>APPSNLMQLPWRQGYSWQPNGAHSNTGSGYPYSSFDASYDWPRWGSATYSVVAAHAGTVRVLSRCQVRVTHPSGWATNYYHMDQIQVSNGQQVSADTKLGVYAGNINTALCEGGSSTGPHLHFSLLYNGAFVSLQGASFGPYRIN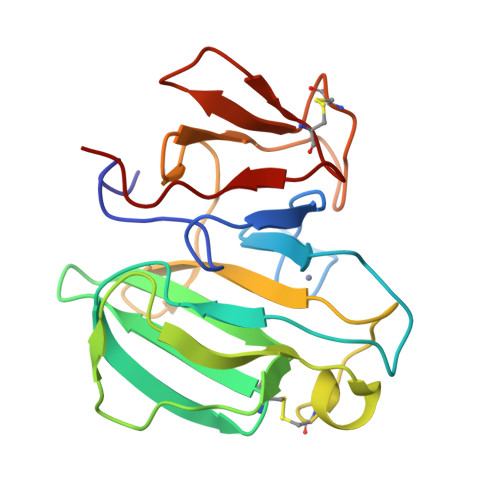VGTSNYDNDCRRYYFYNQSAGTTHCAFRPLYNPGLAL[4x]> MSEWWKEAVVYQIYPRSFYDANGDGFGDLQGVIQKLDYIKNLGADVIWLSPVFDSPQDDNGYDISDYKNMYEKFGTNEDMFQLIDEVHKRGMKIVMDLVVNHTSDEHAWFAESRKSKDNPYRDYYLWKDPKPDGSEPNNWGSIFSGSAWTYDEGTGQYYLHYFSKKQPDLNWENEAVRREVYDVMRFWMDRGVDGWRMDVIPSISKYTDFPDYETDHSRSYIVGRYHSNGPRLHEFIQEMNREVLSHYDCMTVGEANGSDIEEAKKYTDASRQELNMIFTFEHMDIDKEQNSPNGKWQIKPFDLIALKKTMTRWQTGLMNVGWNTLYFENHDQPRVISRWGNDRKLRKECAKAFATVLHGMKGTPFIYQGEEIGMVNSDMPLEMYDDLEIKNAYRELVVENKTMSEKEFVKAVMIKGRDHARTPMQWDAGKHAGFTAGDPWIPV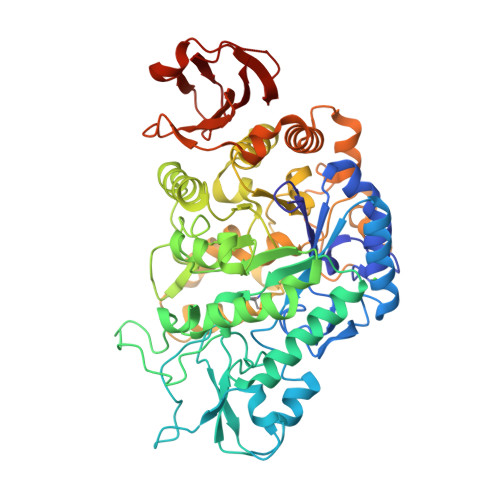NSRYQDINVKESLEDQDSIFFYYQKLIQLRKQYKIMIYGDYQLLQENDPQVFSYLREYRGEKLLVVVNLSEEKALFEAPPELIHERWKVLISNYPQERADLKSISLKPYEAVMGISI>GPGGSPYLITGIPKDPKHPLPIRKDIDDWYLEQTSAGSNRIQLTLFVEALTVIQNRPLNDQLSYFRLAGIHGAPWTEWDGVPGGQKDSKGNPTGFCVHNNYTFPTWHRVYVTLYEQVIYEAMLDFIKQNVPQNGKADWENEAKQWRLPYWDFARFARHGHDN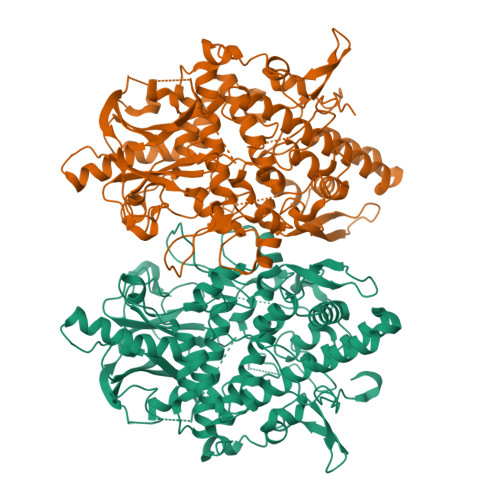TQGDELRLPILVTMPMVKVLVPGQPGKQLSKPNPLYRFQMQTLMGTLERPYAITSQKTEEHGWSFDLPFDKCQSTTKYGLLENYNADVWADGGQNWLRANLALNEHPWYQNLDGWDSVPTLQDMTFRLLTTGGLNWGEFSSTRYDDKKEETQPKNNEQAPKNWMNLEAIHNNVHNWVGGFMFSRPGRHDLKLWGAGHMSSVPVAAYDPIFWLHHCNIDRLTAIWQTVNSGSWFNDDKSKVSKDDDLRPFHRFCEKTRKVVFFRSDDVKDWRSLNYDYAITKDASRIRKEISDLYGQRTKEVYKDFGEEDYILSIRYSRYALGGKPFQINIFFGDVDGKDFYDARSQNFVGSVFNFSGSLEDSNCDKCAQQEQEGVLSVSQLPARLAVHYYKKQNKGEVPTPRYVVVNSQGKAEAEVKVEVALHKTEGTFYDAPARGGSDDYRRVADGKRAEVDDAYRA[4x]>MQQQQLLMSKEIQTNLQVIEENNQRHKAMLDSMQEKFATIIDSSLQSVEEHAKQMHKKLEQLGAMSLPDAEELQNLQEELANERALAQQEDALLESMMMQMEQIKNLRSKNSISMSVHLNKMEESRLTRNHRIDDIKSGIQDYQKLGIEASQSAQAELTSQMEAGMLCLDQGVANCSMLQVHMKNLNQKYEKETNENVGSVRVSGHHHHHH[2x]

Of these, the MT-based motor, Kinesin-5 plays a key role, being essential for the assembly of bipolar spindles in most eukaryotic cells and driving or constraining the rate of spindle elongation. Purified, native Kinesin-5 is a ‘slow’, plus-end-directed, bipolar, homotetrameric motor capable of using pairs of N-terminal motor domains at opposite ends of a central rod to crosslink MTs into bundles. Structure-function analysis of the Drosophila melanogaster Kinesin-5, KLP61F, identified a central bipolar assembly (BASS) domain within the coiled-coil rod that is critical for this motor’s bipolar organization and whose deletion results in disassembled, mostly monomeric, Kinesin-5. Instead of the expected antiparallel arrangement of two side-by-side parallel coiled-coils proposed previously, we find that the BASS domain has a novel four-helix bundle structure, which very likely has important implications for its mechanism of action within the spindle.

The asymmetric unit contains a canonical anti-parallel coiled-coil BASS domain dimer encompassing residues 640–802 of both chains, which represents the basic assembly unit of a Kinesin-5 minifilament. This anti-parallel dimer is associated with a second dimer through a crystallographic dyad axis to form the full tetramer, whose dimer–dimer packing surface extends over a large area (≈7000 Å2) and is stabilized by sequential, alternating hydrophobic and ionic residue interfaces, each occupying three-helical turns. The Kinesin-5 BASS domain is an anti-parallel coiled-coil four-helix bundle that switches polypeptide partners at both ends. Alternating hydrophobic and ionic interfaces specify the assembly of the four BASS monomers to form a rigid central bundle. Each interface occupies approximately three alpha-helical turns on each helix within the bundle, starting at the center with interface A of the BASS tetramer and symmetrically extending toward both ends with paired interfaces B–F. A second striking and unexpected feature revealed by the BASS tetramer structure is the transition from this anti-parallel four-helix central bundle to an asymmetric diamond-shaped four-helix bundle near its ends. This transition promotes a swap in helical organizations, from anti-parallel coiled-coil dimers in the central bundle to parallel coiled-coil dimers at its ends. Near the ends of the bundle, two interfaces mediate these helical swaps: a hydrophobic interface (E) and a di-tyrosine interface (F). Beyond interface F, the N-terminal helices swap organization to form parallel coiled-coils between residues 670–640 stabilized by hydrophobic a and d heptad packing interaction (pCC interface).> GPEKGSEFLKEELHRAQKELKLKDEECERLSKVREQLEQELEELTASLFEEAHKMVR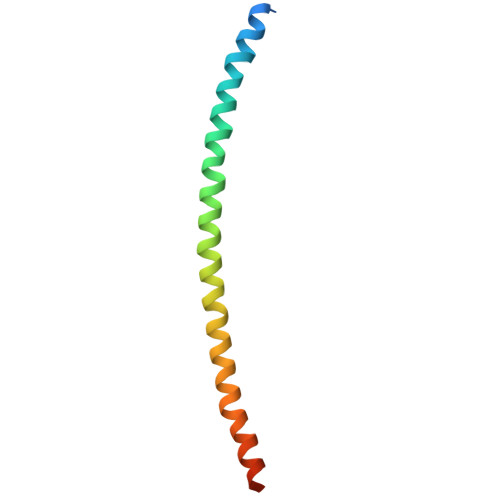EANMKQAASEKQLKEARGKIDMLQAEV> MNMTDDLGGNILLLSGHPGSGKSTIAEALANLPGVPKVHFHSDDLWGYIKHGRIDPWLPQSHQQNRMIMQIAADVAGRYAKEGYFVILDGVVRPDWLPAFTALARPLHYIVLRTTAAEAIERCLDRGGDSLSDPLVVADLHSQFADLGAFEHHVLPVSGKDTDQALQSAINALQSGRFRIDA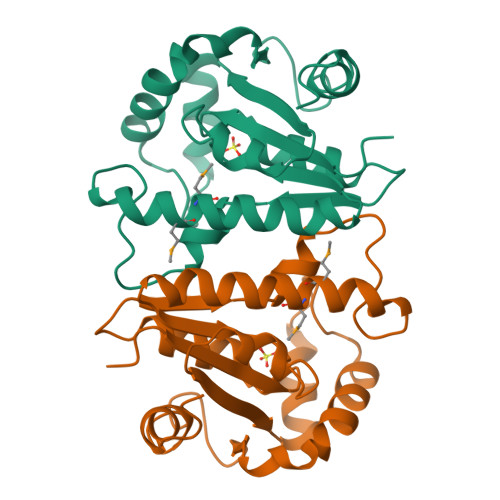SLEHHHHHH>[2x]TPEMPVLENRAAQGDITAPGGARRLTGDQTAALRDSLSDKPAKNIILLIGDGMGDSEITAARNYAEGAGGFFKGIDALPLTGQYTHYALNKKTGKPDYVTDCAASATAWSTGVKTYN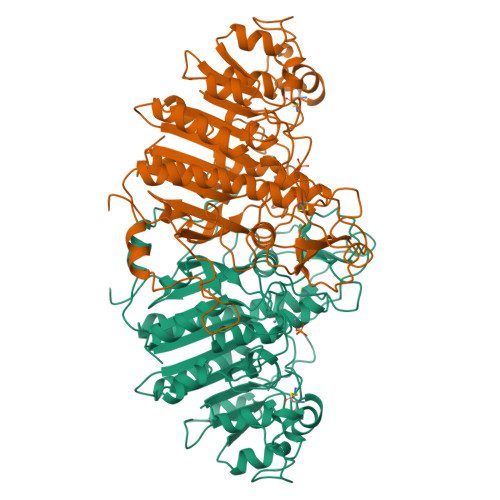GALGVDIHEKDHPTILEMAKAAGLATGNVSTAELQDATPAALVAHVTSRKCYGPSATSEKCPGNALEKGGKGSITEQLLNARADVTLGGGAKTFAETATAGEWQGKTLREQAQARGYQLVSDAASLNSVTEANQQKPLLGLFADGNMPVRWLGPKATYHGNIDKPAVTCTPNPQRNDSVPTLAQMTDKAIELLSKNEKGFFLQVEGASIDKQDHAANPCGQIGETVDLDEAVQRALEFAKKEGNTLVIVTADHAHASQIVAPDTKAPGLTQALNTKDGAVMVMSYGNSEEDSQEHTGSQLRIAAYGPHAANVVGLTDQTDLFYTMKAALGLK>MRILLTNDDGIHAEGLAVLERIARKLSDDVWVVAPETDQSGLAHSLTLLEPLRLRQIDARHFALRGTPTDCVIMGVRHVLPGAPDLVLSGVNSGANMADDVTYSGTVAGAMEGTLLGVRAIALSQEYEYAGDRRIVPWETAEAHAPELIGRLMEAGWPEGVLLNLNFPNCAPEEVKGVRVTAQGKLSHD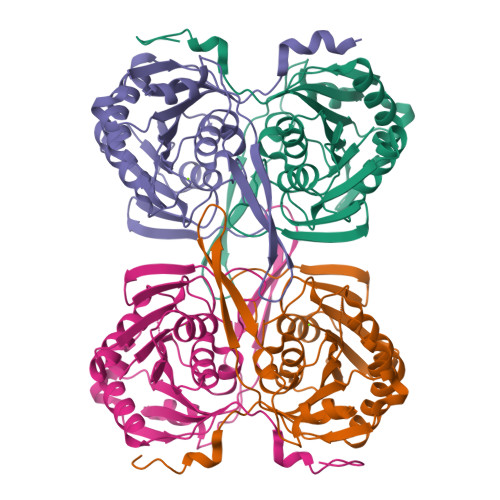ARLDERRDGRGFPYFWLHFGRGKAPVADDSDIAAIRSGCISMTPLHLDLTAHKVRAELGAALGVEALEHHHHHH[4x]>[8x]SFAQYNQVYSTDAANFEHVDHYLTAESWYRPKYILKDGKTWTQSTEKDFRPLLMTWWPDQETQRQYVNYMNAQLGIHQTYNTATSPLQLNLAAQTIQTKIEEKITAEKNTNWLRQTISAFVKT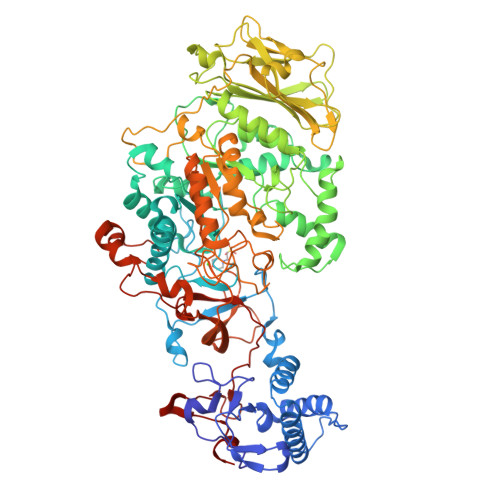QSAWNSDSEKPFDDHLQKGALLYSNNSKLTSQANSNYRILNRTPTNQTGKKDPRYTADRTIGGYEFLLANDVDNSNPVVQAEQLNWLHFLMNFGNIYANDPDANFDSIRVDAVDNVDADLLQIAGDYLKAAKGIHKNDKAANDHLSILEAWSYNDTPYLHDDGDNMINMDNRLRLSLLYSLAKPLNQRSGMNPLITNSLVNRTDDNAETAAVPSYSFIRAHDSEVQDLIRDIIKAEINPNVVGYSFTMEEIKKAFEIYNKDLLATEKKYTHYNTALSYALLLTNKSSVPRVYYGDMFTDDGQYMAHKTINYEAIETLLKARIKYVSGGQAMRNQQVGNSEIITSVRYGKGALKATDTGDRITRTSGVVVIEGNNPSLRLKASDRVVVNMGAAHKNQAYRPLLLTTDNGIKAYHSDQEAAGLVRYTNDRGELIFTAADIKGYANPQVSGYLGVWVPVGAAADQDVRVAASTAPSTDGKSVHQNAALDSRVMFEGFSNFQAFATKKEEYTNVVIAKNVDKFAEWGVTDFEMAPQYVSSTDGSFLDSVIQNGYAFTDRYDLGISKPNKYGTADDLVKAIKALHSKGIKVMADWVPDQMYALPEKEVVTATRVDKYGTPVAGSQIKNTLYVVDGKSSGKDQQAKYGGAFLEELQAKYPELFARKQISTGVPMDPSVKIKQWSAKYFNGTNILGRGAGYVLKDQATNTYFSLVSDNTFLPKSLVNP The TEC family kinase, BTK (Bruton’s tyrosine kinase) is best known as the target of ibrutinib (IMBRUVICA), the first-in-class covalent kinase active site inhibitor used to treat chronic lymphocytic leukemia, mantle cell lymphoma, Waldenström’s macroglobulinemia, and chronic graft-versus-host disease. The TEC and SRC kinases share the SH3–SH2–kinase domain arrangement (the ‘Src module’). In contrast, BTK contains an extended N-terminal region (PHTH–PRR) consisting of the phospholipid-binding Pleckstrin homology (PH) domain followed by a Tec homology (TH) domain and a long linker housing two proline-rich regions (PRR). Membrane-induced dimerization activates BTK and we present here a crystal structure of an activation loop swapped BTK kinase domain dimer that likely represents the conformational state leading to trans-autophosphorylation. Together, these data provide the first structural elucidation of full-length BTK and allow a deeper understanding of allosteric control over the BTK kinase domain during distinct stages of activation.

The crystallization construct used to capture this new conformation of the BTK kinase domain included mutation of Y551E to mimic the phosphorylated activation loop, mutation of L390G to disfavor autoinhibitory contacts, and dasatinib bound to the active site. The kinase domain forms a face-to-face dimer in the crystal with two intermolecular interfaces; the β3/C-helix loop in the N-lobe forms one interface and the domain swapped activation loop and G-helix mediate an extensive interface between the C-lobes. The activation loop of one monomer in the face-to-face BTK dimer structure extends into the active site of the other monomer but electron density is missing for residues 546–559, which includes the Y551 autophosphorylation site. Nevertheless, superimposing two different substrate-bound kinase structures (tyrosine and serine phosphoacceptors) onto the BTK kinase domain shows that Y551 from one BTK kinase domain monomer would easily reach a viable phosphor-acceptor position in the active site of the opposing monomer. The swapped BTK dimer structure may therefore represent a conformation along the trans-autophosphorylation activation pathway. The canonical Lys/Glu salt bridge with active kinase domains does not form in the BTK kinase domain dimer due to the unusual conformation of the phenylalanine side of the DFG motif (F540). The F540 side chain intercalates between the Lys/Glu side chains adopting what has previously been termed ‘DFG-up’ or ‘DFGinter’. The C-helix is therefore held in an intermediate state between the C-helix in and C-helix out conformations associated with active and inactive kinases, respectively.

>MKNAPSTAGGGYGSWEIDPKDLTFLKELGTGQFGVVKYGKWRGQYDVAIKMIREGSMSEDEFIEEAKVMMNLSHEKLVQLYGVCTKQRPIFIITEYMANGCLLNYLREMRHRFQTQQLLEMCKDVCEAMEYLESKQFLHRDLAARNCLVNDQGVVKVSDFGLSRYVLDDEETSSVGSKFPVRWSPPEVLMYSKFSSKSDIWAFGVLMWEIYSLGKMPYERFTNSETAEHIAQGLRLPRPHLASERVYTIMYSCWHEKADERPSFKILLSNILDVMDEES[2x]> MGNEVAGVEDISVEIKPSSKRNSDARRTSRNVCSNEERKRRKYFHMLYLVCLMVHGFIRNEWINSKRLSRKLSNLVPEKVFELLHPQKDEELPLRSTRKLLDGLKKCMELWQKHWKITKKYDNEGLYMRTWKEIEMSANNKRKFKTLKRSDFLRAVSKGHGDPDISVQGFVAMLRACNVNARLIMSCQPPDFTNMKIDTSLNGNNAYKDMVKYPIFWCEVWDKFSKKWITVDPVNLKTIEQVRLHSKLAPKGVACCERNMLRYVIAYDRKYGCRDVTRRYAQWMNSKVRKRRITKDDF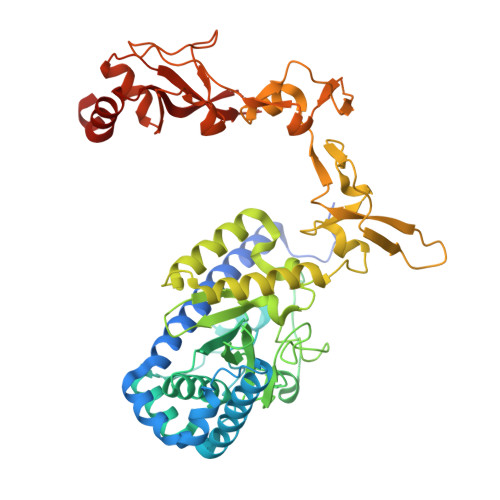GEKWFRKVITALHHRKRTKIDDYEDQYFFQRDESEGIPDSVQDLKNHPYYVLEQDIKQTQIVKPGCKECGYLKVHGKVGKVLKVYAKRDIADLKSARQWYMNGRILKTGSRCKKVIKRTVGRPKGEAEEEDERLYSFEDTELYIPPLASASGEITKNTFGNIEVFAPTMIPGNCCLVENPVAIKAARFLGVEFAPAVTSFKFERGSTVKPVLSGIVVAKWLREAIETAIDGIEFI> TDALNVLLIIVDDLRPSLGCYGDKLVRSPNIDQLASHSLLFQNAFAQQAVAAPSRVSFLTGRRPDTTRLYDFNSYWRVHA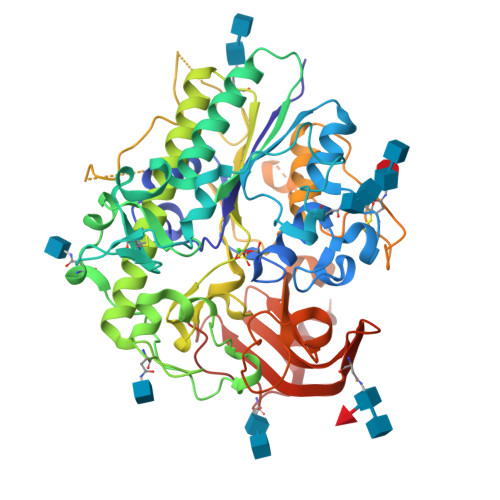GNFSTIPQYFKENGYVTMSVGKVFHPGISSNHTDDSPYSWSFPPYHPSSEKYENTKTCRGPDGELHANLLCPVDVLDVPEGTLPDKQSTEQAIQLLEKMKTSASPFFLAVGYHKPHIPFRYPKEFQKLYPLENITLAPDPEVPDGLPPVAYNPWMDIRQREDVQALNISVPYGPIPVDFQRKIRQSYFASVSYLDTQVGRLLSALDDLQLANSTIIAFTSDHGWALGEHGEWAKYSNFDVATHVPLIFYVPGRTASLPEAGEKLFPYLDPFDSASQLMEPGRQSMDLVELVSLFPTLAGLAGLQVPPRCPVPSFHVELCREGKNLLKHFRFRDLEEDPYLPGNPRELIAYSQYPRPSDIPQWNSDKPSLKDIKIMGYSIRTIDYRYTVWVGFNPDEFLANFSDIHAGELYFVDSDPLQDHNMYNDSQGGDLFQLLMP> MHHHHHHHHGGSEFSIDGGSLEVLFQGPSSPSHQIWLPPLDVPPTLDELLPPLSPSAAHGYTADGWEWRGRLHAVVGLVDRPFDQRRDPYWLDLSGGAGHVGVAGGPQTGKSTML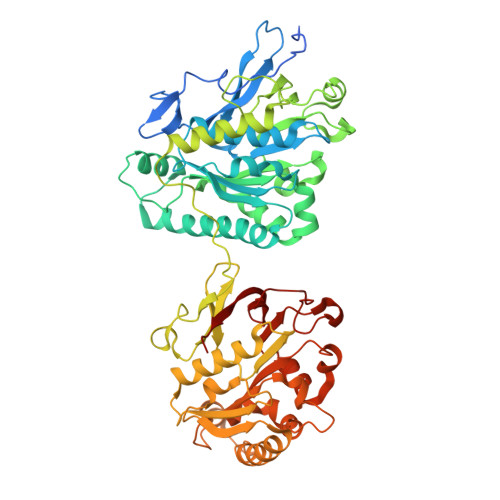RTLITSLALLHTPQEVQFYCLDFGGGTLAGLAELPHVGSVATRLDADRIRRTVAEVSALLEQREQEFTERGIDSMATYRRLRATGEYAGDGFGDVFLVVDNWLTLRQDYEALEDSITQLAARGLGYGIHVVLSSNKWSEFRTSIRDLLGTKLELRLGDPYESEVDRKKAANVPENRPGRGLTRDGYHFLTALPRIDGDTSAETLTEGIATTVKTIREAWHGPTAPPVRMLPNVLPAAQLPSAAESGTRIPIGIDEDSLSPVYLDFNTDPHFLVFGDTECGKSNLLRLITAGIIERYTPQQARLIFIDYSRSLLDVATTEHQIGYAASSTAASSLVRDIKGAMEARLPPPDLTPEQLRSRSWWTGAELFLVVDDYEMVATSDNPLRPLAELLPQARDIGLHLIIARSMGGAGRALYEPIIQRIKEMASPGLVMSGNKDEGILLGNVKPHKLPQGRGYFVERRSGTRLIQTAYRES> PPKWKVKKQKLAEKAAREAELTAKKAQARQALSIYLNLPTLDEAVNTLKPWWPGLFDGDTPRLLACGIRDVLLEDVAQRNIPLSHKKLRRAMKAITRSESYLCAMKAGACRYDTEGY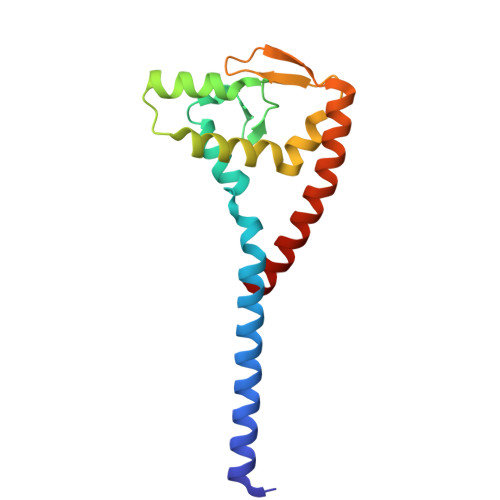VTEHISQEEEVYAAERLDKIRRQNRIKAELQAVLD3-(pyridin-3-yl)prop-2-yn-1-yl 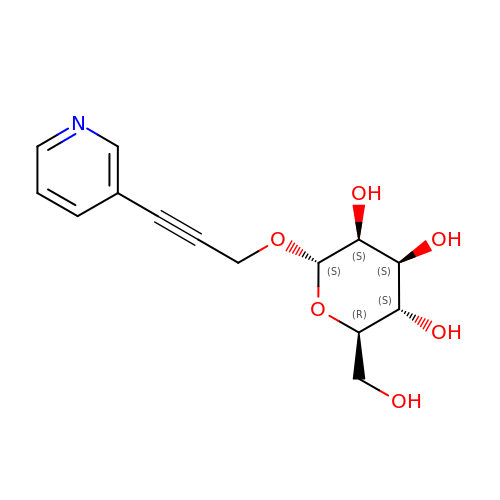alpha-D-mannopyranoside | C14 H17 N O6 | GMPRLXFHQUHVDW-DGTMBMJNSA-N>[2x]LTLGNTTSSVILTNYMDTQYYGEIGIGTPPQTFKVVFDTGSSNVWVP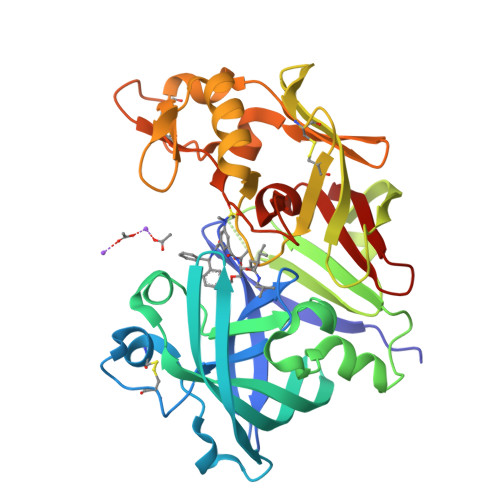SSKCSRLYTACVYHKLFDASDSSSYKHNGTELTLRYSTGTVSGFLSQDIITVGGITVTQMFGEVTEMPALPFMLAEFDGVVGMGFIEQAIGRVTPIFDNIISQGVLKEDVFSFYYNRDSENSQSLGGQIVLGGSDPQHYEGNFHYINLIKTGVWQIQMKGVSVGSSTLLCEDGCLALVDTGASYISGSTSSIEKLMEALGAKKRLFDYVVKCNEGPTLPDISFHLGGKEYTLTSADYVFQESYSSKKLCTLAIHAMDIPPPTGPTWALGATFIRKFYTEFDRRNNRIGFALARH> QCSQFLRGQ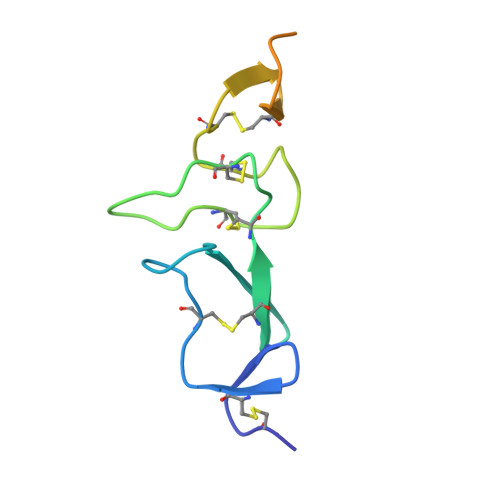ECVEECRVLQGLPREYVNARHCLPCHPECQPQNGSVTCFGPEADQCVACAHYKDPPFCVARCPSGVKPDLSYMPIWKFPDEEGACQPC>[3x]MAQLALQMSSLGVEGEGIWLALGTIGMLLGMLYFIADGLDVQDPRQKEFYVITI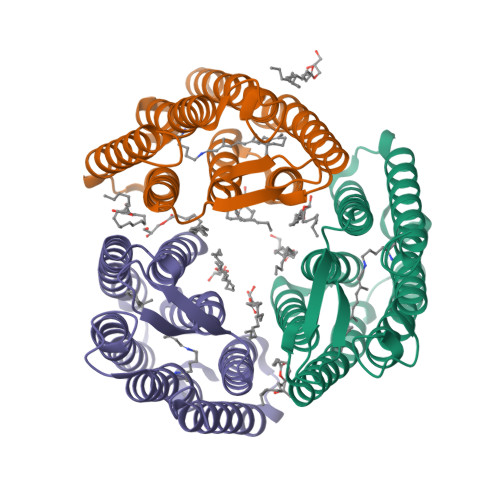LIPAIAAASYLSMFFGFGLTEVSLANGRVVDVYWARYADWLFTTPLLLLDIGLLAGASQRDIGALVGIDAFMIVTGLVATLTKVVVARYAFWTISTISMVFLLYYLVAVFGEAVSDADEDTRSTFNALRNIILVTWAIYPVAWLVGTEGLALTGLYGETLLFMVLDLVAKVGFGFILLRSRAIMGGGSEPTPSAQETAADLVPRGSLEHHHHHH> MASENYLNHPTFGLLYQICSFGD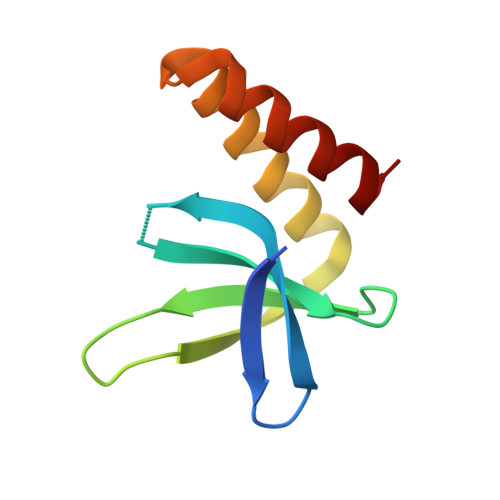SKELFATLYAQRLFFLVAFDARGTRFEPIGRNEARMLVDNRLRQLRRDASLQEYNQLQQVFKQTFL(2~{R})-~{N}-[5-(5-azanylpyridin-3-yl)-4-ethanoyl-1,3-thiazol-2-yl]piperazine-2-carboxamide | C15 H18 N6 O2 S | 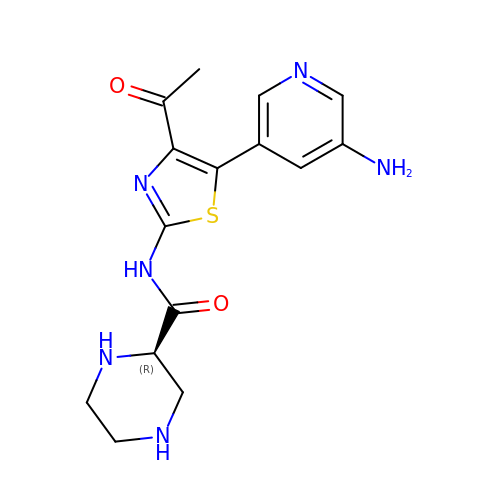CTUFUQNJXFRTNL-LLVKDONJSA-N> MELKFSAEVELTLSREVDPAEIEPTVEEFVKEANEDLLQRGVPTGKEGAKIESYYVLYDTIYMEITGTRYLRPHEAAMRVRKRLAERLGRKHRVGVRDLKIPRYEVVLRFDREVTYDYVGYVPVADDVVVEDGTVRLTFQDVDEEMLRRHVIDRVIRLVAWAVEERSELVERVTKVEPGTVVDESGPRRIRFRGDVTEEARRRGWVKEFPGRGQWIYTPPMAALFEVLRDFLLERVTRKLGFEPALFPKLIPLETMFRMRYLHGLPDGMYYVCPPKRDPEL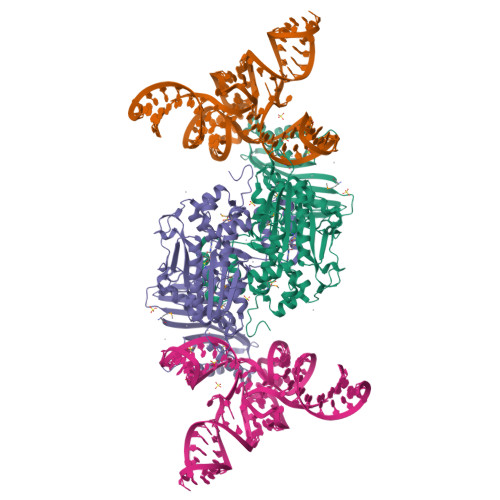FDDFKRELYVWGELNERTLGSLKEKLRDPGYVLAPAQCEPFYELLRDEVVDPERLPIKLYDCSGWTYRWEGGAAKGLERVNEFQRIEHVWIAEPEEAYRIRRELLEATKRVAEELELEWKVVVSDDPFYLEGRLLEDRDIELPDVPSYEFEVYLPFKGERSSEEAWISVGSFNVHGEHFVDGFNVKEKSGRTLFTGCAGLGVTRWVVGLLAQHGFYPYEWPEPILERIDEKFGGLPEVPKTLTWPE>[2x]GIDPFTHMPVSVQQSLAAYNQRKADLVNRSIAQMREATTLANGVLASLNLPAAIEDVSGDTVPQSILTKSRSVIEQG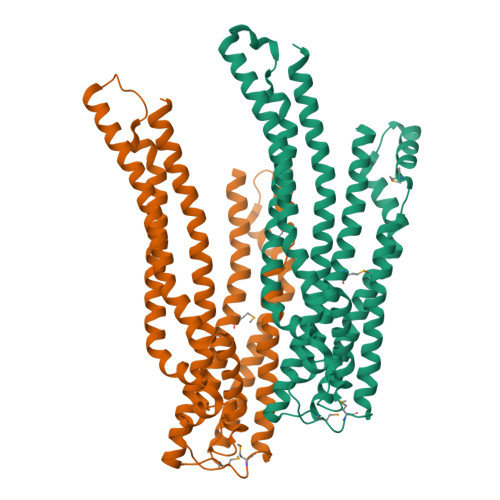GIQTVDQLIKELPELLQRNREILDESLRLLDEEEATDNDLRAKFKERWQRTPSNELYKPLRAEGTNFRTVLDKAVQADGQVKECYQSHRDTIVLLCKPEPELNAAIPSANPAKTMQGSEVVNVLKSLLSNLDEVKKEREGLENDLKSVNFDMTSKFLTALAQDGVINEEALSVTELDRVYGGLTTKVQESLKKQEGLLKNIQVSHQEFSKMKQSNNEANLREEVLKNLATAYDNFVELVANLKEGTKFYNELTEILVRFQNKCSDIVFARKTER>MALAPITAPDITSICKDASSGIGNQEGAIRTRKCCPPSLGKKIKDFQFPNDKKVRMRWPAHKGTKKQVDDYRRAIAAMRALPDDDPRSFVSQAKIHCAYCNGGYTQVDSGFPDIDIQIHNSWLFFPFHRWYLYFYERI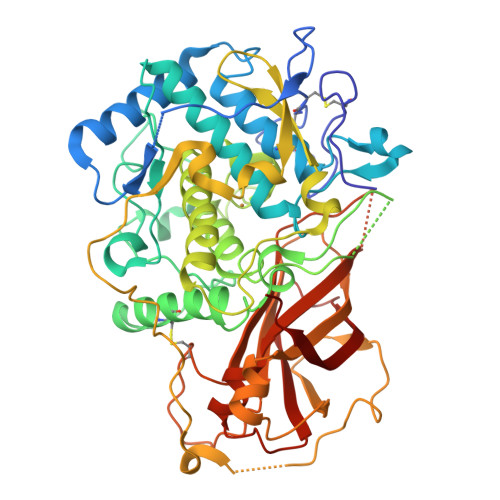LGSLIDEPNFALPYWKWDEPKGMPISNIFLGDASNPLYDQYRDANHIEDRIVDLDYDGKDKDIPDQQQVACNLSTVYRDLVRNGVDPTSFFGGKYVAGDSPVANGDPSVGSVEAGSHTAVHRWVGDPTQPNNEDMGNFYSAGYDPVFYIHHANVDRMWKLWKELRLPGHVDITDPDWLNASYVFYDENKDLVRVYNKDCVNLDKLKYNFIENSKEVFPWRNSRPPQRRKSAQVATTGDVKTVEQTKFPVRLNQIFKVRVKRPAVNRTEEEKDQANEVLLIKKIKYDSGKFVKFDVFVNDKLKDGVFTTPCDPEYAGGFAQIPHNDKRSMVMTSTARFGLNELLEDTNTEGEEYATVTLVPRTGCEDLTVGEIKIELVPIPKA[8x]> MEARAHGALPNNYDRERFINGVGGDDKALKRKLEEPLSDITKELDTVIAQSDVAVADPKGQLCPDADVPDEMEHITDGILPLNLLLIRLAEFSHSKLEELVTMLASKPVPQHAVNGNGSH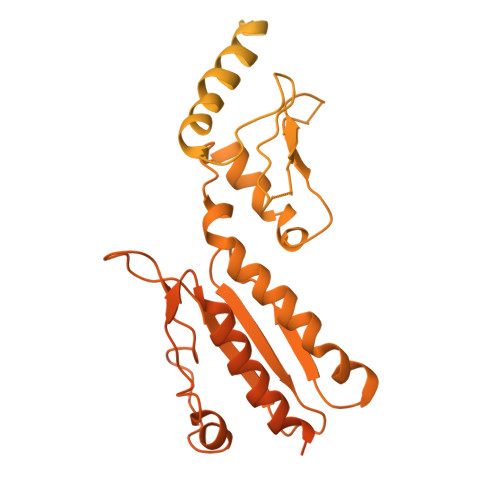STLVEDASPESQEKKRLLLNTIQDLHSRWVKALVITEWARNAEKVGKLIDIRTHLFKKLELYPQVLNDFINLKRDMAWAKVPSPDLKTALHILTHGEVTWMPDFNFLDPPPLTTEETLRWINDMNLALHARLQLEEHDKLPPPFKNYTIDSGRVTFRVRGEFEVDLSISEEDFSEQFWFINFRFDFSPAPAELTPAVRYWMTEKVNNILKTEGLGGCYKYLHEFTLTQKIAELHRQAIALNKGRWANSLRVEKLNRNLGIHYWANRLHSQNLKSWIIIGVHSGEDPQGLEEPKPSYLMVQWFREGVEQFIDIPFSQEKLSIEEILEFVTAKHVGYLLFSLFRKFDGKPRFTQGKKARLELNVWTQKPEDYYLSMQLLDDEDLKIQVNPWMGDFITTPSTGPWNRTLNSLGNPAEEGSKELENFRYIYIISVLKAQGKSHGWSVVRSPISQDELRSIVHSESASSRETFQAAWTRFVDWDPQWYAMRSMSLAGDQWWLVEVTSQRQSISGNRLVFFTKMAPCFSEERLTDGFFNGLRDHSRRLIAEITNLRELYPGITPSQLRKLIDPTRQPPVLPVKASKILGDFGGADAQSIAWLKDPVWLIYRGSACDTRVSDSPQQKRTQPVLDVFEAYLDVTDRRRFQTLNPRLDRDILYNPYTGRFMFRLRAKMGVPVVPLLGIRVRQLQRLLDFLEGLRRVGDDAVPERVTLREIVFSYGATRKRDSTNQPKVRPWRVRLDLTKEEGVGVVLEKGNPHLRVINRLEDLVNSQKFYSLATYLTLSLPLFRAFQQLENAWQTAQENGRGSCFILHLSLDKHTIRFVLPGHQRQISLLIQPHEKEGKLVWEVGRPRHDPELLNENCEFNRVLKERVWTISGSGFKGLVTGAAAEPDEGIERLLVLISDAVLHLSTSQPATAPPQPPQAQPSQQVQQVQQQQVVSQLQPQAQQPRSAMPHASVGQQQPHGAPAPMARFPPQQQQIFQQQRPPQPQPNMHGGQISQPNMHGGPKPQLQGQHGQPGQMVAAPQQQGQRPGTGTAAGMGRSNAPLVVLD>[10x]MQEGQNRKTSSLSILAIAGVEPYQEKPGEEYMNEAQLAHFRRILEAWRNQLRDEVDRTVTHMQDEAANFPDPVDRAAQEEEFSLELRN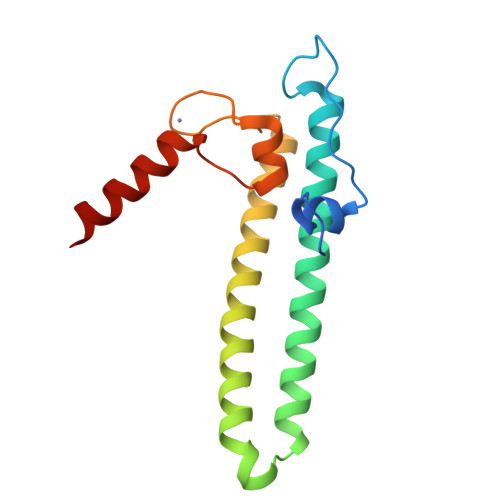RDRERKLIKKIEKTLKKVEDEDFGYCESCGVEIGIRRLEARPTADLCIDCKTLAEIREKQMAG> TRQFLIYNEDHKR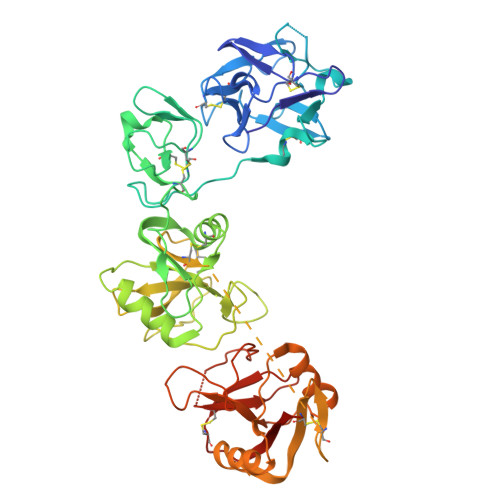CVDAVSPSAVQTAACNQDAESQKFRWVSESQIMSVAFKLCLGVPSKTDWVAITLYACDSKSEFQKWECKNDTLLGIKGEDLFFNYGNRQEKNIMLYKGSGLWSRWKIYGTTDNLCSRGYEAMYTLLGNANGATCAFPFKFENKWYADCTSAGRSDGWLWCGTTTDYDTDKLFGYCPLKFEGSESLWNKDPLTSVSYQINSKSALTWHQARKSCQQQNAELLSITEIHEQTYLTGLTSSLTSGLWIGLNSLSFNSGWQWSDRSPFRYLNWLPGSPSAEPGKSCVSLNPGKNAKWENLECVQKLGYICKKGNTTLNSFVIPSESDVPTHCPSQWWPYAGHCYKIHRDEKKIQRDALTTCRKEGGDLTSIHTIEELDFIISQLGYEPNDELWIGLNDIKIQMYFEWSDGTPVTFTKWLRGEPSHENNRQEDCVVMKGKDGYWADRGCEWPLGYICKMKSHHHHHH Azolopyrimidine | C12 H9 Cl N4 O | 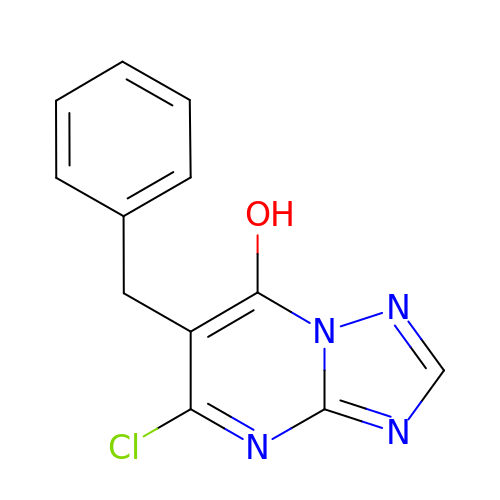AFMPXANNRQOFLA-UHFFFAOYSA-N>MSKLAAFGGPPAVPRDRRHVEWPLVEDEDRKAVIDALDGARLVSNSDGENPVSTLEEQWAGRFGFGHCVAVSTGTAALSLALAALGVGPGDEVIVPALSFIATGLAPVHQMAVPVFADVDPVTFNLDPDDVERRITGRTAAIIPVHLHGAPADMDRITAIARRHGLAVIEDAAQAPGATHRGRPVGGIGDAGAFSLQATKNIPTCGEGGLLVTGNAELAESVRRGRQFGEVIESGRERDYVSYGLGWNHKMNALQAAFTSAQLTRFDDYESARQRNVAAFLARLAELPGLRVPTAAPDTTHAWHILRFRFDPAAFGLDGVRPQALRSALRRLLRAEGVPMSQYQLMPLPDQKVFVDRVGFGGGYPWTVTGATGPAAGEDHPVA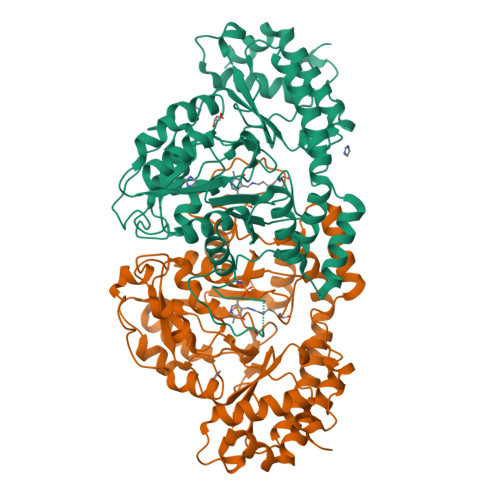RAVIADSLTLQKRHLHPESGELLHLYADAFEKVWANPDMVATLAGAASGGHHHHHH[2x]>GSHMACTWPAWEHFKRAYISDGGRVIDPSDARKITTSEGQSYALFFALAADDRPMFDNVLEWTKDNLAQGDPGEHLPAWLWGKKDENNWTVLDSNSASDADIWIAWSLLEAGRLWKEARYTTLGNALLNRIAKEEVVTVPGLGPMLLPGKVGFAEETVWRLNPSYLPPQIARYLTRFGEPWTTLQETNHRLLLETAPKGFSPDWVRYEKSKGWQLAPDKTLISGYAAIRVYLWVGMMNDHDAQKASLLERLKPMAALTAKKGVVPEKVDVATA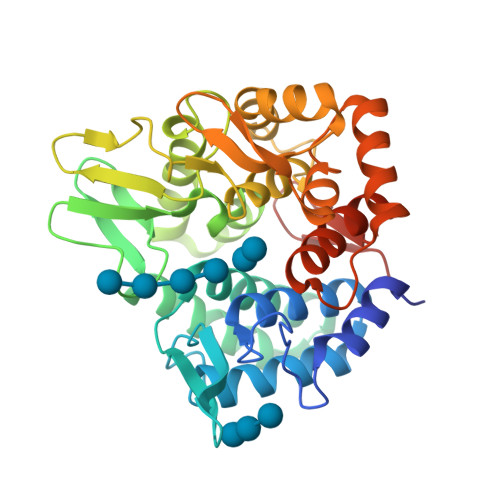QPRGDGPVGFAAALLPFLQDRDAQAVQRQKVADHFPGDDAYFSYVLTLFGQGWDEHRFRFTPRGELQPDWGQACASSQ[4x]>[2x]GHMETIHVGDRCLCRPGDRLGSVRFVGRVASL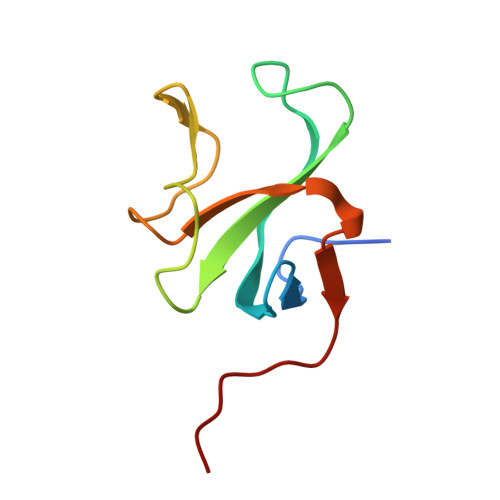KPGYWVGVEFDEPVGKGDGTVKGTRVFQCQPNYGGFLRPDQVEVGDFPPEVF>GSSHHHHHHSSGLVPRGSMSTSWSDRLQNAADMPANMDKHALKKYRREAYHRVFVNRSLAMEKIKCFGFNMDYTLAVYKSPEYESLGFELTVERLVSIGYPQELLSFAYDSTFPTRGLVFDTLYGNLLKVDAYGNLLVCAHGFNFIRGPETREQYPNKFIQRDDTERFYILNTLFNLPETYLLACLVDFFTNCPRYTSCETGFKDGDLFMSYRSMFQDVRDAVDWVHYKGSLKEKTVENLEKYVVKDGKLPLLLSRMKEVGKVFLATNSDYKYTDKIMTYLFDFPHGPKPGSSHRPWQSYFDLILVDARKPLFFGEGTVLRQVDTKTGKLKIGTYTGPLQHGIVYSGGSSDTICDLLGAKGKDILYIGDHIFGDILKSKKRQGWRTFLVIPELAQELHVWTDKSSLFEELQSLDIFLAELYKHLDSSSNERPDISSIQRRIKKVTHDMDMCYGMMGSLFRSGSRQTLFASQVMRYADLYAAS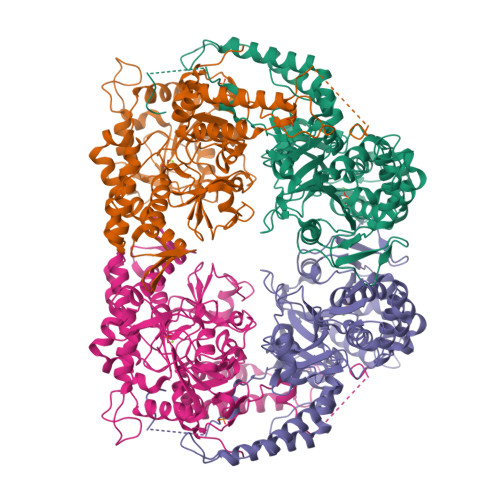FINLLYYPFSYLFRAAHVLMPHESTVEHTHVDINEMESPLATRNRTSVDFKDTDYKRHQLTRSISEIKPPNL[2x]> SHKKLVINKDMRTDL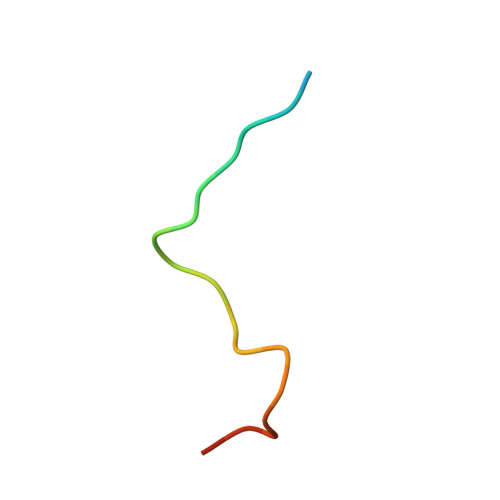FSPPNKD> SNAMPSENPIGKTMKSIDEQSLHNARRLFESGDIDRIEVGTTAGLQQIHRYLFGGLYDFAGQIREDNISKGGFRFANAMYLKEALVKIEQMPERTFEEIIAKYVEMNIAHPFLEGN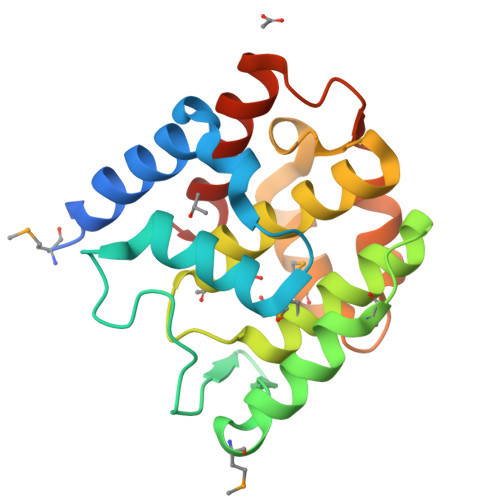GRSTRIWLDLVLKKNLKKVVNWQNVSKTLYLQAMERSPVNDLELRFLLKDNLTDDVDNREIIFKGIEQSYYYEGYEKG>GSHMIEVVCNDRLGKKVRVKCNTDDTIGDLKKLIAAQTGTRWNKIVLKKWYTIFKDHVSLGDYEIHDGMNLELYYQ[6x];>SLSIEETNKLRAKLGLKPL[6x]

Although structurally very similar to ubiquitin, the highly conserved protein Hub1 does not function as a covalent modifier but binds proteins only non-covalently. Hub1 of yeast and mammalian cells associates with the spliceosome through interaction with the tri-snRNP protein Snu66. Comprising solely the ubiquitin-fold and lacking N- or C-terminal extensions, Hub1 is only able to function through non-covalent interactions with other proteins. Importantly, Hub1 does not seem to influence splicing of all splice substrates equally, but to facilitate only certain splicing events of particular introns/exons of pre-mRNAs. These findings thus lead to the model that the ubiquitin-like protein Hub1 plays a conserved role in the spliceosome as modulator of splicing activity.

To characterize the Hub1–HIND interaction further, we obtained structural information of human Hub1 in complex with a peptide corresponding to the single human HIND sequence. The interaction between Hub1 and the α-helical HIND peptide is mediated through a salt bridge formed by D22 of Hub1 and R127 of HIND, strengthened by hydrophobic contacts involving aliphatic fragments of residues of hSnu66’s HIND and the Hub1 interface. Although Hub1 possesses an ubiquitin fold, it uses the opposite protein surface for Snu66 binding compared to ubiquitin for binding to ubiquitin receptors like Rad23. In contrast, the Hub1–HIND interaction surface is located on the opposite side to the canonical UBD patch formed by helix α1 and sheets β1β2. The X-ray analysis revealed that human and S. cerevisiae Hub1-HIND complexes have overall very similar, superimposable structures with a root mean squared deviation (RMSD) of 0.716 Å. The two structures only show small differences, particularly in protein loops extending opposite of the Hub1–HIND interaction surface. Because RS domains can mediate protein–protein interactions as well, we mapped the Hub1-binding site using hSnu66 truncations and found that the single HIND motif of hSnu66 is sufficient and necessary for Hub1 binding. Testing the relevance of the salt bridge between D22 of Hub1 and R127 of the HIND element for this interaction, we found that a recombinant fusion protein of GFP with the N-terminal domain of hSnu66 (aa 1–139), but not a similar fragment bearing an alanine replacement of a the R127 residue (R127A) in its HIND domain, bound endogenous Hub1 of human cell extracts in GFP-immunoprecipitation assays. Conversely, only immunoprecipitation of stably expressed GFP-fusions of wild-type (WT) Hub1 but not of a Hub1 variant harboring an alanine replacement of the D22 residue (D22A) co-isolated endogenous hSnu66 from human cell lysates. From these findings we infer that binding of human Hub1 to Snu66 does indeed depended on the integrity of this salt bridge, showing that physical properties of Hub1 are highly conserved at the molecular level.>ATAAEIAALPRQKVELVDPPFVHAHSQVAEGGPKVVEFTMVIEEKKIVID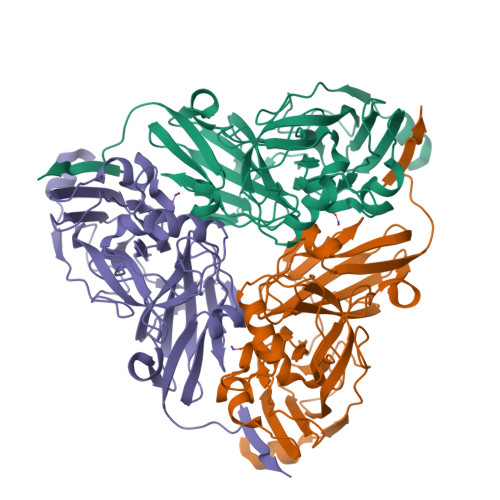DAGTEVHAMAFNGTVPGPLMVVHQDDYLELTLINPETNTLMHNIDFHAATGALGGGGLTEINPGEKTILRFKATKPGVFVYHCAPPGMVPWHVVSGMNGAIMVLPREGLHDGKGKALTYDKIYYVGEQDFYVPRDENGKYKKYEAPGDAYEDTVKVMRTLTPTHVVFNGAVGALTGDKAMTAAVGEKVLIVHSQANRDTRPHLTGGHGDYVWATGKFNTPPDVDQETWFIPGGAAGAAFYTFQQPGIYAYVNHNLIEAFELGAAAHFKVTGEWNDDLMTSVLAPSGTIEGR[3x]> MQADILDGKQKRVNLNSKRLVNCNQVDVNQLVPIKYKWAWEHYLNGCANNWLPTEIPMGKDI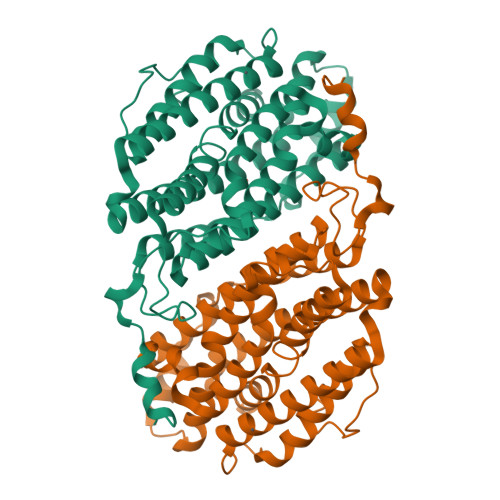ELWKSDRLSEDERRVILLNLGFFSTAESLVGNNIVLAIFKHVTNPEARQYLLRQAFEEAVHTHTYLYICESLGLDEKEIFNAYNERAAIKAKDDFQMEITGKVLDPNFRTDSVEGLQEFVKNLVGYYIIMEGIFFYSGFVMILSFHRQNKMIGIGEQYQYILRDETIHLNFGIDLINGIKEENPEIWTPELQQEIVELIKRAVDLEIEYAQDCLPRGILGLRASMFIDYVQHIADRRLERIGLKPIYHTKNPFPWMSETIDLNKEKNFFETRVIEYQHAASLTW>MAAALLARASGPARRALCPRAWRQLHTIYQSVELPETHQMLLQTCRDFAEKELFPIAAQVDKEHLFPAAQVKKMGGLGLLAMDVPEELGGAGLDYLAYAIAMEEISRGCASTGVIMSVNNSLYLGPILKFGSKEQKQAWVTPFTSGDKIGCFALSEPGNGSDAGAASTTARAEGDSWVLNGTKAWITNAWEASAAVVFASTDRALQNKGISAFLVPMPTPGLTLGKKEDKLGIRGSSTANLIFEDCRIPKDSILGEPGMGFKIAMQTLDMGRIGIASQALGIAQTALDCAVNYAENRMAFGAPLTKLQVIQFKLADMALALESARLLTWRAAMLKDNKKPFIKEAAMAKLAASEAATAISHQAIQILGGMGYVTEMPAERHYRDARITEIYEGTSEIQRLVIAGHLLRSYRS[4x]

Here we report the use of single particle cryo-EM to identify multiple proteins from three enriched heterogeneous fractions prepared from human liver mitochondrial lysate. Using this approach, we were able to simultaneously identify and solve cryo-EM structures of nine different human mitochondrial enzymes: short chain acyl-CoA dehydrogenase (SCAD), medium chain acyl-CoA dehydrogenase (MCAD), isovaleryl-CoA dehydrogenase (IVD), delta (3, 5)-delta dienoyl-CoA isomerase (ECH1), aspartate aminotransferase (GOT2), glutamate dehydrogenase (GLUD1), mitochondrial superoxide dismutase 2 (SOD2), catalase (CAT), and mitochondrial aldehyde dehydrogenase (ALDH2). Functionally, the three acyl-CoA dehydrogenases—SCAD, MCAD and IVD—are involved in beta oxidation and amino acid catabolism. Finally, SOD2, CAT, and ALDH2 are all involved in clearing toxic byproducts of oxidative respiration.

Butanoyl-CoA and other four or five carbon fatty acid acyl-CoA molecules are the initial substrates of SCAD. We obtained a high-resolution 3.15 Å structure of SCAD bound to substrate and cofactor using 16,677 single particle cryo-EM projections. The global fold of SCAD is a tetramer made up of a dimer of dimers. Each individual monomeric unit contains a β-sheet core flanked by N-terminal and C-terminal α-helical domains. The FAD cofactor-binding site is at the intersection of the three domains of each monomer. Additionally, the flavin ring interacts with the C-terminal domain of the corresponding subunit in each dimer set. The ligand-binding site lies parallel to cofactor and the catalytic site E392. Residues F152, L154, N207, F261, M265, L268, D269, R272, I342, I397, and the catalytic E392 residue form the substrate cavity. Mutations in the corresponding SCAD gene can lead to SCAD deficiency (SCADD), a rare autosomal recessive disorder.> MVSLTFKNFKKEKVPLDLEPSNTILETKTKLAQSISCEESQIKLIYSGKVLQDSKTVSECGLKDGD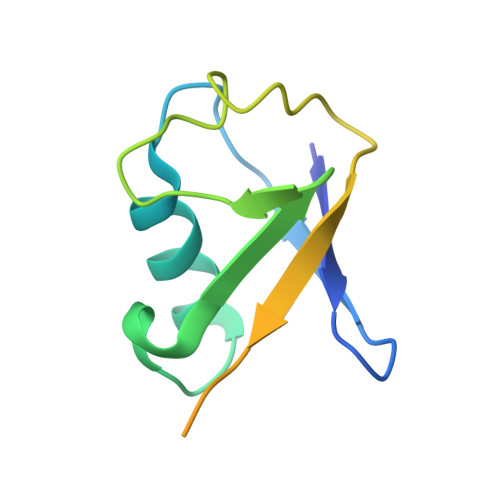QVVFMVSQKKSTKTKVTERDPNSSSVDKLAAALEHHHHHH> SNAQKLIKDLYVDKEWSADYQPFRIAGNLYYIGTYDLGMFLITTPKGHILINTGVAGSDTLIKAHMKTLGFKFKDIRILLTTHAHYDHVGAMAAVKQQTHAKMMVNEKDAALLADGGNSDYVMGGKG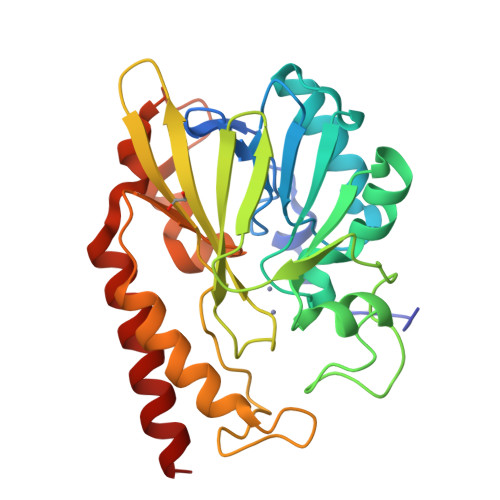SMFLPVKADRLLHDGDSIQLGGMKIVMRQHPGHTPGANSFLFDVKDAVRTYKVLIANIPSILNDTKLSGMPLYPEVGKDYAYTLKAMKALKFDLWLAPHAGQYELHKKHQPGDAYNPAAFSDRAGYDDVLDEWQQIYDKRVKEE>[2x]MSEYDKYSTPLSSRYASEEMSKIFSLRNRFSTWRKLWLNLAIAEKEVGL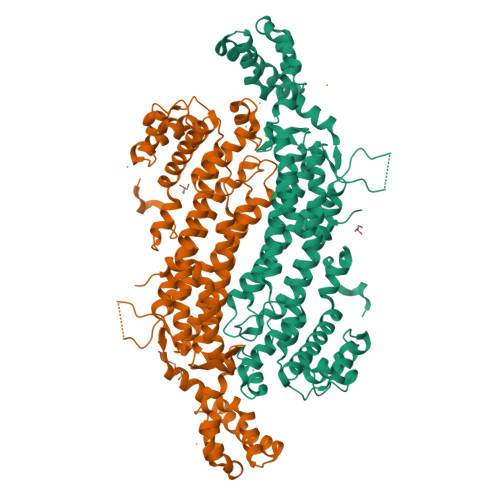SVITDEAIEQMKQHLEITDKEIQDAAVEEAKVRHDVMAHVHVFGETCPSAAGIIHLGATSCFVTDNADLIFLRDAYDVLIPKLVNVIDRLSKFALEYKDLPVLGWTHFQPAQLTTVGKRATLWLQELLWDLRNMVRARNDIGLRGVKGTTGTQASFLSLFHGDHDKVEELDKRVVELLGFDIVYPVTGQTYSRKIDIDVLSPLASFGATAHKFATDIRLLANLKEIEEPFEKSQIGSSAMAYKRNPMRCERVCSLARHLGGLFNDAVQTASVQWFERTLDDSAIRRISLPSAFLTVDILLSTMLNITSGLVVYPKVIERRINSELPFMATENIIMAMVEKGGSRQDCHEEIRVLSHQASAVVKQEGGDNDLIERIKSTEYFKPIWNDLDTLLDPKTFVGRAPQQTEKFVKNDVANALKPFEKYITTENVALKV3'-deoxy-3'-[(L-alpha-glutamyl)amino]adenosine 5'-(dihydrogen phosphate) | C15 H22 N7 O9 P | 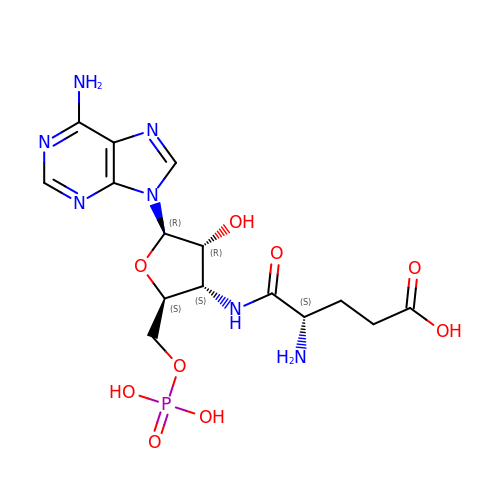SDRBGGWQNQDMBH-HQMNMZSFSA-N> GAMTFTRYSRLRVIAEIRHGDIFHSANIVSSIEFDRDDELFATAGVSRCIKVFD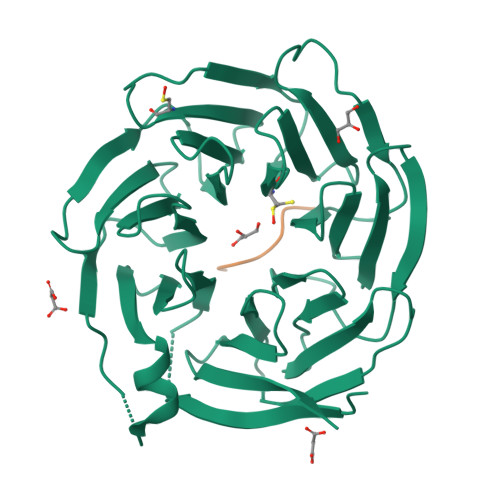FSSVVNEPADMQCPIVEMSTRSKLSCLSWNKHEKNHIASSDYEGIVTVWDVTTRQSLMEYEEHEKRAWSVDFSRTEPSMLVSGSDDCKVKVWCTRQEASVINIDMKANICCVKYNPGSSNYIAVGSADHHIHYYDLRNISQPLHVFSGHKKAVSYVKFLSNNELASASTDSTLRLWDVKDNLPVRTFRGHTNEKNFVGLTVNSEYLACGSETNEVYVYHKEITRPVTSHRFGSPDMDDAEEEAGSYFISAVCWKSDSPTMLTANSQGTIKVLVLAA;> XEDQMVPSITY2-[2-(2-CYCLOHEXYL-2-GUANIDINO-ACETYLAMINO)-ACETYLAMINO]-N-(3-MERCAPTO-PROPYL)-PROPIONAMIDE 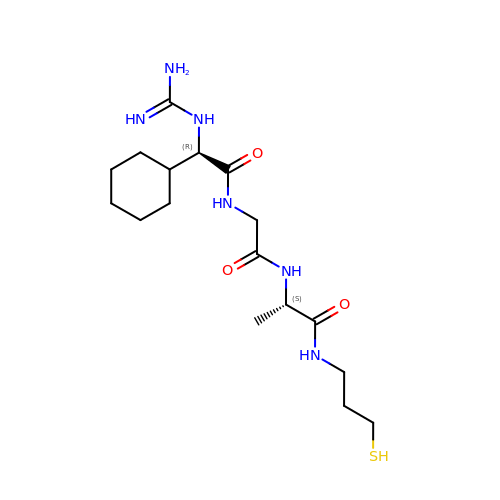| C17 H32 N6 O3 S | YLLNYDDZOMCFDE-SMDDNHRTSA-N> MPA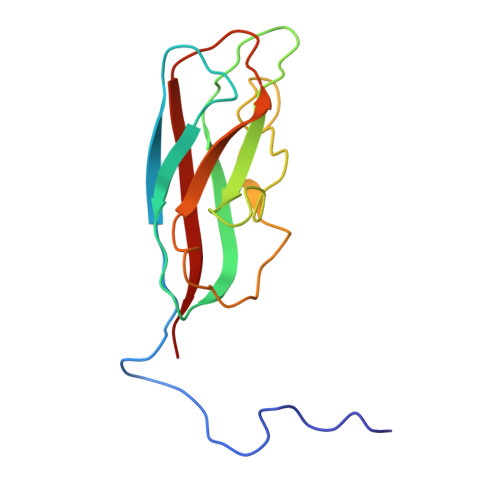TNSAQARLAAPGHGFGGNVKVSYGSVAFTGTITTADAATVCNLPVGAIVLGVTLESDDLDTNATPTITLNVGDAGSATRYFSASTVAQAGTSSSAPATTGLLWTVTEGNTAVRIAVANNAATSADGSVRVAVTYYLP> MSLFKARDWWSTVLGDKEEFDQGCLCLADVDNTGNGQDKIIVGSFMGYLRIFNPHPVKTGDGAQAEDLLLEVHLRDPILQVEVGKFVSGTEMLHLAVLHSRKLCVYSVSGTLGNVEHGNQYQIKLMYEHNLQRTACNMTYGSFGGVKGRDLICIQSVDGMLMVFEQESYAFGRFLPGSLLPGPLAYSSRTDSFITVSSCHQVESYKYQVLAFATDADKRQETEQQKHGSGKRLVVDWTLNIGEQAIDICIVSFIQSASSVFVLGERNFFCLKDNGQIQFMKKLDYSPSCFLPYCSVSEGTINTLIGNHNNMLHIYQDVTLKWATQLPHVPVAVRVGCLHDLKGVIVTLSDDGHLQCSYLGTDPSLFQAPKVESRELNYDELDMELKELQKVIKNVNKSQDVWPLTEREDDLKVSAMVSPNFDSVSQ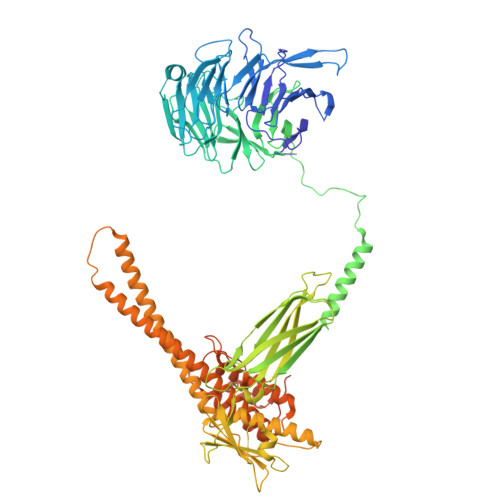ATDVEVGADLVPSVTVKVTLKNRVALQKIKLSIYVQPPLVLTGDQFTFEFMAPEMTRTVGFSVYLKGSYSPPELEGNAVVSYSRPTERNPDGIPRVSQCKFRLPLKLVCLPGQPSKTASHKLTIDTNKSPVSLLSLFPGFAKQSEDDQVNVMGFRFLGGSQVTLLASKTSQRYRIQSEQFEDLWLITNELIIRLQEYFEKQGIKDFTCSFSGSVPLEEYFELIDHHFELRINGEKLEELLSERAVQFRAIQRRLLTRFKDKTPAPLQHLDTLLDGTYKQVIALADAVEENQDNLFQSFTRLKSATHLVILLIGLWQKLSADQIAILEAAFLPLQQDTQELGWEETVDAALSHLLKTCLSKSSKEQALNLNSQLGIPKDTSQLKKHITLFCDRLAKGGRLCLSTDAAAPQTMVMPGGCATIPESDLEGRSIDQDSSELFTNHKHLMVETPVPEVSPLQGVTE>TGRGVKYWFCYGTKCYYFIMNKTTWSGCKANCQHYSVPIVKIEDEDELKFLQRHVIPEGYWIGLSYDKKKKEWAWIDNGPSKFDM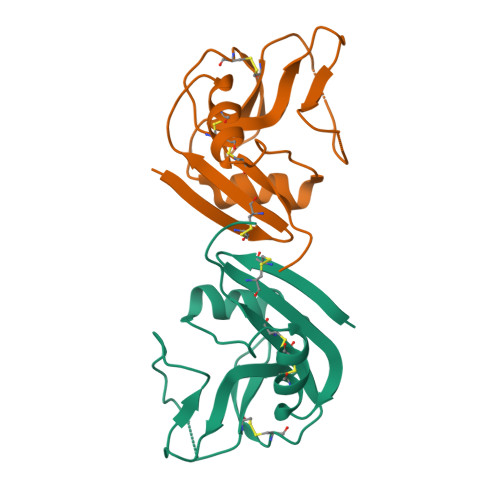KIRKMNFKSRGCVFLSKARIEDTDCNIPYYCICGKKLDKFPD[2x]> SMENKNLNYILGLALGIASVGWAVVEIDEKENPLRLIDVGVRTFERAEVPKTGESLALSRRLARSARRLTQRRVARLKKAKRLLKSENILLSTDERLPHQVWQLRVEGLDHKLERQEWAAVLLHLIKHRGYLSQRKNESKSENKELGALLSGVDNNHKLLQQATYRSPAELAVKKFEVEEGHIRNQQGAYTHTFSRLDLLAEMELLFSRQQHFGNPFASEKLLENLTALLMWQKPALSGEAILKMLGKCTFEDEYKAAKNTYSAERFVWITKLNNLRIQENGLERALNDNERLALMEQPYDKNRLFYSQVRSILKLSDEAIFKGLRYSGEDKKAIETKAVLMEMKAYHQIRKVLEGNNLKAEWAELKANPTLLDEIGTAFSLYKTDEDISAYLAGKLSQPVLNALLENLSFDKFIQLSLKALYKLLPLMQQGLRYDEACREIYGDHYGKKTEENHHFLPQIPADEIRNPVVLRTLTQARKVINGVVRLYGSPARIHIETGREVGKSYKDRRELEKRQEENRKQRENAIKEFKEYFPHFAGEPKAKDILKMRLYKQQNAKCLYSGKPIELHRLLEKGYVEVDAALPFSRTWDDSFNNKVLVLANENQNKGNLTPFEWLDGKHNSERWRAFKALVETSAFPYAKKQRILSQKLDEKGFIERNLNDTRYVARFLCNFIADNMHLTGEGKRKVFASNGQITALLRSRWGLAKSREDNDRHHALDAVVVACSTVAM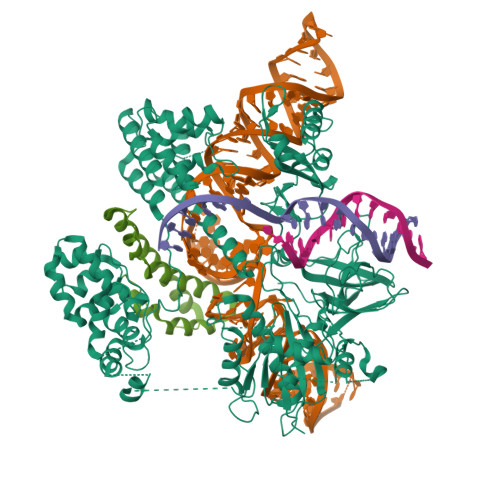QQKITRFVRFEAGDVFTGERIDRETGEIIPLHFPTPWQFFKQEVEIRIFSDNPKLELENRLPDRPQANHEFVQPLFVSRMPTRKMTGQGHMETVKSAKRLNEGISVIKMPLTKLKLKDLELMVNREREKDLYDTLKARLEAFNDDPAKAFAEPFIKKGGAIVKSVRVEQIQKSGVLVREGNGVADNASMVRVDVFTKGGKYFLVPIYTWQVAKGILPNKAATQYKDEEDWEVMDNSATFKFSLHPNDLVKLVTKKKTILGYFNGLNRATGNIDIKEHDLDKSKGKQGIFEGVGIKLALSFEKYQVDELGKNIRLCKPSKRQPVR;> SMKITSSNFATIATSENFAKLSVLPKNHREPIKGLFKSAVEQFSSARDFFKNENYSKELAEKFNKEAVNEAVEKLQKAIDLAEKQGIQF> ALTNLVAEPFAKLEQDFGGSIGVYA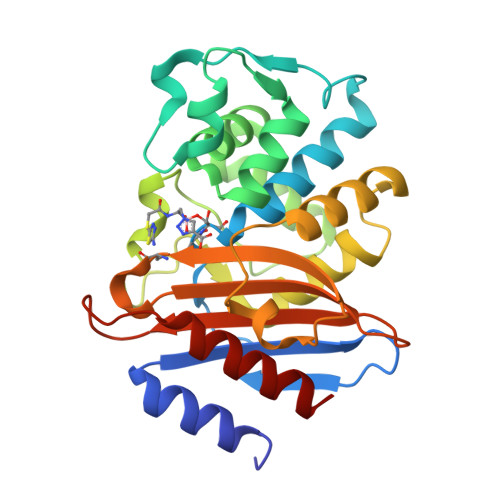MDTGSGATVSYRAEERFPLCSSFKGFLAAAVLARSQQQAGLLDTPIRYGKNALVPWSPISEKYLTTGMTVAELSAAAVQYSDNAAANLLLKELGGPAGLTAFMRSIGDTTFRLDRWELELNSAIPGDARDTSSPRAVTESLQKLTLGSALAAPQRQQFVDWLKGNTTGNHRIRAAVPADWAVGDKTGTCGVYGTANDYAVVWPTGRAPIVLAVYTRAPNKDDKHSEAVIAAAARLALEGLG> MGSQVSTQRSGSHENSNSATEGSTINYTTINYYKDSYAATAGKQSLKQDPDKFANPVKD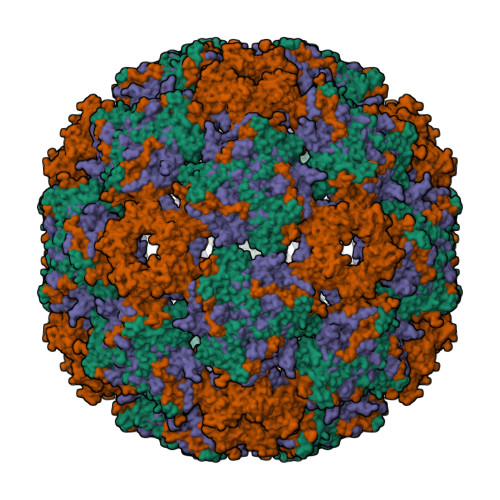IFTEMAAPLKSPSAEACGYSDRVAQLTIGNSTITTQEAANIIVGYGEWPSYCSDSDATAVDKPTRPDVSVNRFYTLDTKLWEKSSKGWYWKFPDVLTETGVFGQNAQFHYLYRSGFCIHVQCNASKFHQGALLVAILPEYVIGTVAGGTGTEDSHPPYKQTQPGADGFELQHPYVLDAGIPISQLTVCPHQWINLRTNNCATIIVPYINALPFDSALNHCNFGLLVVPISPLDYDQGATPVIPITITLAPMCSEFAGLRQAVTQ;> GDRVADVIESSIGDSVSRALTRALPAPTGQNTQVSSHRLDTGKVPALQAAEIGASSNASDESMIETRCVLNSHSTAETTLDSFFSRAGLVGEIDLPLEGTTNPNGYANWDIDITGYAQMRRKVELFTYMRFDAEFTFVACTPTGGVVPQLLQYMFVPPGAPKPDSRESLAWQTATNPSVFVKLSDPPAQVSVPFMSPASAYQWFYDGYPTFGEHKQEKDLEYGACPNNMMGTFSVRTVGTSKSKYPLVVRIYMRMKHVRAWIPRPMRNQNYLFKANPNYAGNSIKPTGASRTAITTL;> GFPTELKPGTNQFLTTDDGVSAPILPNFYPTPCIHIPGEVRNLLELCQVETILEVNNVPTNATSLMERLRFPVSAQAGKGELCAVFRADPGRSGPWQSTLLGQLCGYYTQWSGSLEVTFMFTGSFMATGKMLIAYTPPGGPLPKDRATAMLGTHVIWDFGLQSSVTLVIPWISNTHYRAHARDGVFDYYTTGLVSIWYQTNYVVPIGAPNTAYIIALAAAQKNFTMKLCKDASDILQTGTIQ>[3x]MDRNSLSNSLKTCYKYLNQTSRSFAAVIQALDGEMRNAVCIFYLVLRALDTLEDDMTISVEKKVPLLHNFHSFLYQPDWRFMESKEKDRQVLEDFPTISLEFRNLAEKYQTVIADICRRMGIGMAEFLDKHVTSEQEWDKYCHYVAGLVGIGLSRLFSASEFEDPLVGEDTERANSMGLFLQKTNIIRDYLEDQQGGREFWPQEVWSRYVKKLGDFA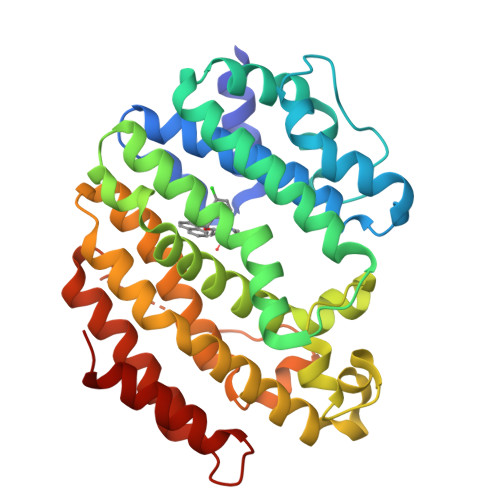KPENIDLAVQCLNELITNALHHIPDVITYLSRLRNQSVFNFCAIPQVMAIATLAACYNNQQVFKGAVKIRKGQAVTLMMDATNMPAVKAIIYQYMEEIYHRIPDSDPSSSKTRQIISTIRTQN>MGHHHHHHHHHHHMAQGTLIRVTPEQPTHAVCVLGTLTQLDICSSAPEDCTSFSINASPGVVVDIAHGPPAKKKSTGSSTWPLDPGVEVTLTMKVASGSTGDQKVQISYYGPKTPPVKALLYLTGVEISLCADITRTGKVKPTRAVKDQRTWTWGPCGQGAILLVNCDRDNLESSAMDCEDDEVLDSEDLQDMSLMTLSTKTPKDFFTNHTLVLHVARSEMDKVRVFQATRGKLSSKCSVVLGPKWPSHYLMVPGGKHNMDFYVEALAFPDTDFPGLITLTISLLDTSNLELPEAVVFQDSVVFRVAPWIMTPNTQPPQEVYACSIFENEDFLKSVTTLAMKAKCKLTICPEEENMDDQWMQDEMEIGYIQAPHKTLPVVFDSPRNRGLKEFPIKRVMGPDFGYVTRGPQTGGI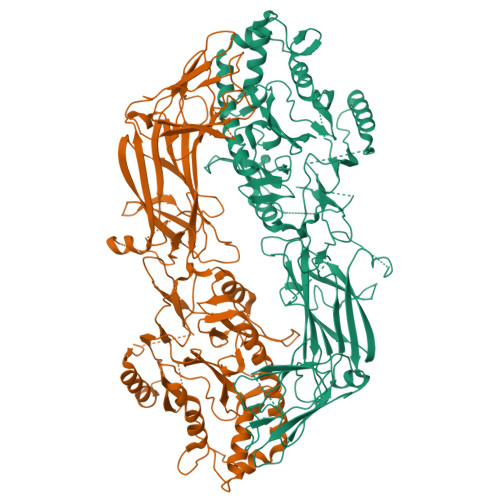SGLDSFGNLEVSPPVTVRGKEYPLGRILFGDSCYPSNDSRQMHQALQDFLSAQQVQAPVKLYSDWLSVGHVDEFLSFVPAPDRKGFRLLLASPRSCYKLFQEQQNEGHGEALLFEGIKKKKQQKIKNILSNKTLREHNSFVERCIDWNRELLKRELGLAESDIIDIPQLFKLKEFSKAEAFFPNMVNMLVLGKHLGIPKPFGPVINGRCCLEEKVCSLLEPLGLQCTFINDFFTYHIRHGEVHCGTNVRRKPFSFKWWNMVP[2x]>SALAQRPGSVSKWVRLNVGGTYFLTTRQTLCRDPKSFLYRLCQADPDLDSDKDETGAYLIDR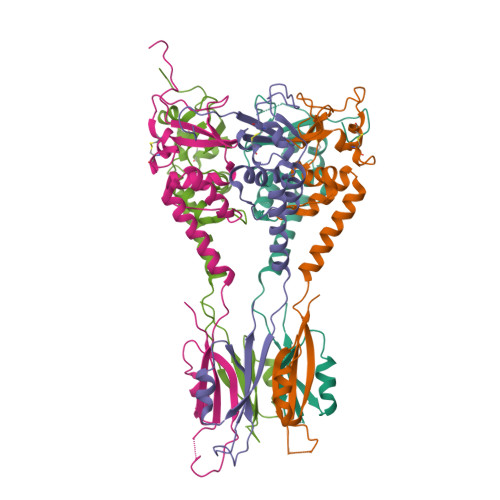DPTYFGPVLNYLRHGKLVINKDLAEEGVLEEAEFYNITSLIKLVKDKIRERDSKTSQVPVKHVYRVLQCQEEELTQMVSTMSDGWKFEQLVSIGSSYNYGNEDQAEFLCVVSKELHNTPYGTASEPSEKAKILQERGSRM[5x]> AADIFSKFKKDMEVKFAQEFGSNKQTGGDITDKTAKFLRLGPEQDPRKVEMIKAGKEIAEKRGIAFYNPMMHSGAPLGQRAITPYTISGTDIVCEPDDLHYVNNAAMQQMWDDIRRTCIVGLDMAHETLEKRLGKEVTPETINHYLEVLNHAMPGAAVVQEMMVETHPALVDDCYVKVFTGDDALADEIDKQFLIDINKEFSEEQAAQIKASIGKTSWQAIHIPTIVSRTTDGAQTSRWAAMQIGMSFISAYAMCAGEAAVADLSFAAKHAALVSMGEMLPARRARGPNEPGGLSFGHLSDIVQTSRVSEDPAKIALEVVGAGCMLYDQIWLGSYMSGGVGFTQYATAAYTDDILDNNTYYDVDYINDKYNGAATVGKDNKVKASLEVVKDIATESTLYGIETYEKFPTALEDHFGGSQRATVLAAAAGVACSLATGNANAGLSGWYLSMYLHKEAWGRLGFFGFDLQDQCGATNVLSYQGDEGLPDELRGPNYPNYAMNVGHQGGYAGIAQAAHSGRGDAFTVNPLLKVCFADDLLPFNFAEPRREFGRGAIREFVPAGERSLVIPA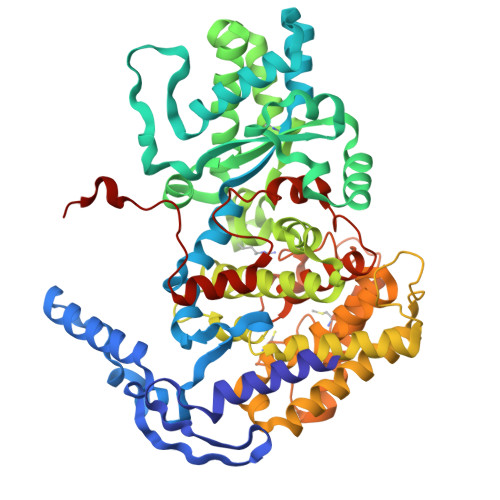K> TQKSLSKEEIERYSRQMIVPGMGKEGQLRLMNAKVLIIGAGGLGCPAAQYLAGAGVGTIGIVDGDSVETSNLHRQVAHATKRVGMLKVDSLITHLIEINPLPVYVPYRFDLTPQNAAQIIKPWDVILDCTDNPATRYLISDVCVLLGKPLVSAASVQKSGQLIVLNCPPTPQGVVNKKAAPCYRCCFKKPPPPSAQTSKGEAGIMGPVVGMMGVAQAGEAIKILVSQLHMPPKEGEEVSPEKNLVQPTLLIYTYDLNSAIGPYSFRALKMGGRKKDCFACGENSTLTLDGIKSGNPNYVQF;> IPITVDFSGGLEMLFDNQRRHSISLPAKDTEGKPVTIAFLIDYICKKLMKDPRTDLFVLDNHIRPGILVLINDADWELEGEEAYEIQPNDNILFVSTLHGG

In eukaryotes, the ubiquitin‐related modifier 1 (Urm1) pathway is responsible for the synthesis of 2‐thiolated wobble uridine (U34). Uba4 is a two‐domain protein containing an adenylation domain (AD) and a rhodanese‐like domain (RHD), which are both essential for the dual function of Uba4 in sulfur transfer and ubiquitin‐like conjugation (Furukawa et al, 2000; Huang et al, 2008; Schmitz et al, 2008; Leidel et al, 2009; Noma et al, 2009). Uba4 activates the C‐terminus of Urm1 via an ATP‐dependent adenylation step, receives mobilized sulfur from the Nfs1/Tum1‐relay system by its RHD, and subsequently forms thiocarboxylated Urm1 (Urm1‐COSH; Leidel et al, 2009; Noma et al, 2009). We heterologously expressed and purified Uba4 from Chaetomium thermophilum (CtUba4), a thermophilic fungus harboring highly stable proteins, well‐suited for X‐ray crystallography and other in vitro approaches (Bock et al, 2014).

Therefore, we generated a Uba4C202K mutation to convert the labile thioester intermediate into a non‐hydrolysable iso‐peptide bond between the activated C‐terminus of Urm1 and the ε‐amino group of the introduced lysine. The covalently linked Uba4C202K–Urm1 complex formed well‐diffracting crystals resulting in a structure at 3.15 Å resolution, and its atomic model was refined to R/Rfree values of 21.1%/26.2%. The structure revealed two Urm1 molecules with slightly higher B‐factors bound to a dimer of the Uba4 AD (Figs 3B and EV3A), while no specific density could be attributed to the RHD, which although present in our crystals, appears to be mobile at this specific reaction step. In contrast to Uba4 alone, the Uba4–Urm1 dimer is fully symmetric and the AD interface falls on a twofold crystallographic axis. Interestingly, the C‐terminal GG‐motif of Urm1 is positioned in the same groove that was occupied by the linker region in the unbound Uba4 structure (Figs 3D and EV3B). Importantly, a helical region localized adjacent to the ATP‐binding site (aa 72–88) in the structure of apo Uba4 becomes disordered and flexible in the structure of the Uba4–Urm1 complex (Fig EV4). In contrast, the loop containing Cys202, known as “crossover loop” in other E1 enzymes, becomes structured in the Uba4–Urm1 complex and an electron density can be clearly assigned to the covalent peptide bond between the introduced Lys202 and the C‐terminal glycine (Gly111) of Urm1 (Fig EV3B). Hence, the crossover loop acts as a clamp toward the C‐terminus of Urm1, which appears to remain virtually identically bound to the AD throughout all reaction steps, including adenylation, thioester formation, and possibly thiocarboxylation. Therefore, the Uba4C202K‐Urm1 structure represents a unique previously uncharacterized reaction step, mimicking the thioester formation after the release of AMP that can serve as a model for this reaction intermediate in all other E1‐UBL and SCP systems.> MAKTRPGVASKIKTGRKELDSYTIKGTNKVVRAGD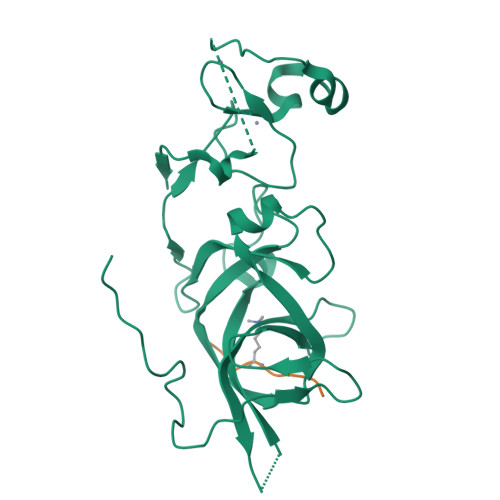CVLMRPSDAGKPPYVARVEKIEADARNNVKVHCRWYYRPEESLGGRRQFHGAKELFLSDHFDVQSAHTIEGKCIVHTFKNYTRLENVGAEDYYCRFEYKAATGAFTPDRVAVYCKCEMPYNPDDLMVQCEGCKDWYHPACVGMTIEEAKKLDHFVCAECSSDDDVAASQNGFTSSPADDVKVRLSLFSHLLYRCSITYL;> LATKAARKSAPATGGV> MGSSHHHHHHSQDPNSMGKLTLLLLAILVWLQYSLWFGKNGIHDYTRVNDDVAAQQATNAKLKARNDQLFAEIDDLNGGQEALEERARNELSMTRPGETFYRLVPDASKRAQSAGQNNR;> MISRVTEALSKVKGSMGSHERHALPGVIGDDLLRFGKLPLCLFICIILTAVTVVTTAHHTRLLTAQREQLVLERDALDIEWRNLILEENALGDHSRVERIATEKLQMQHVDPSQENIVVQK;> MSQAALNTRNSEEEVSSRRNNGTRLAGILFLLTVLTTVLVSGWVVLGWMEDAQRLPLSKLVLTGERHYTRNDDIRQSILA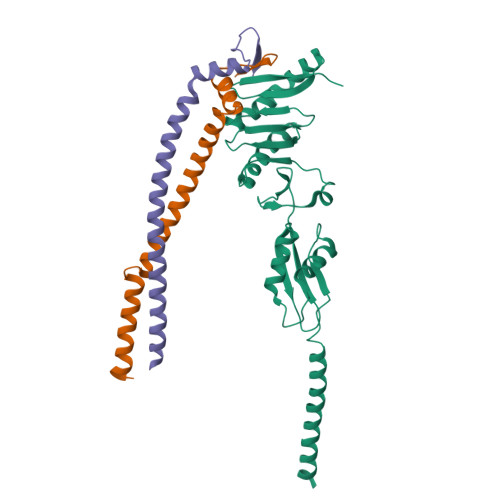LGEPGTFMTQDVNIIQTQIEQRLPWIKQVSVRKQWPDELKIHLVEYVPIARWNDQHMVDAEGNTFSVPPERTSKQVLPMLYGPEGSANEVLQGYREMGQMLAKDRFTLKEAAMTARRSWQLTLNNDIKLNLGRGDTMKRLARFVELYPVLQQQAQTDGKRISYVDLRYDSGAAVGWAPLPPEESTQQQNQAQAEQQ>[4x]GMTTSEHIAALTALVETYVMAMTRGDRPALERIFFGKASEVGHYEGELLWNSRDAFIA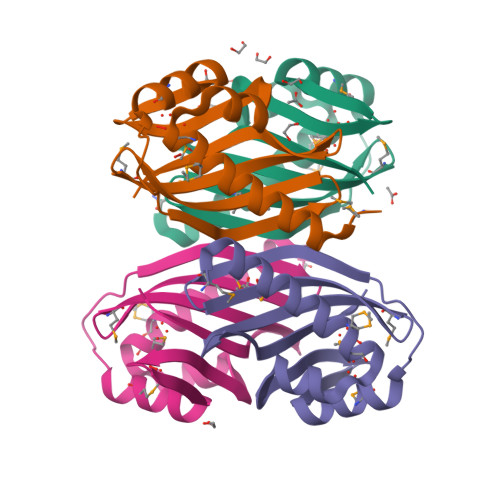MCEDAADAETDPFWAISSVSVQGDIAMLHVENDWAGMRFDDFLTVLLHEGSWRIVSKVYRIR Second, the ribonucleoprotein telomerase elongates shortened telomeres at chromosomal ends using a reverse transcriptase activity. Although the human telomerase holoenzyme is composed of multiple accessory subunits, catalysis is localized to the telomerase reverse transcriptase (TERT) subunit. We found that, in terms of global protein structure, minimal rearrangement is required to proceed through the catalytic cycle.

Throughout the TERT catalytic cycle, we observed that Y256 rests in the minor groove of the DNA and is in position to clash with the 2’-OH of an incoming rNTP. Therefore, we hypothesized this residue to be the steric gate in telomerase. Compared to WT TERT, the insertion of a matched rGTP by Y256A showed a 1,490-fold increase in kpol to 5.5 s−1 and a 12-fold decrease in Kd to 73 μM. Thus, the sugar selectivity of TERT dropped from 14,000-fold between rGTP and dGTP for WT TERT to less than 2-fold for the Y256A TERT variant. To test for structural rearrangements, we crystallized the pre-nucleotide binary state of TERT Y256A (state A6), and saw minimal structural differences compared to the WT protein. The position of the primer terminus was not changed, and catalytic residues D251, D343, and D344 were in position to catalyze the nucleotidyl transferase reaction. Upon closer examination of the active site pocket, the substitution of Y256 with alanine resulted in a more open nucleotide binding pocket. The distance from the C2 carbon of the dGpCpp to residue 256 shifted from 3.3 Å in WT TERT to 5.7 Å in TERT Y256A, showing that the TERT Y256A has much more room to accommodate the 2’-OH. Taken as a whole, these results indicate Y256 clashes with the 2’-OH of rNTPs to provide sugar discrimination and is the steric gate in telomerase.

> GMVHYYRLSLKSRQKAPKIVNSKYNSILNIALKNFRLCKKHKTKKPVQILALLQEIIPKSYFGTTTNLKRFYKVVEKILTQSSFECIHLSVLHKCYDYDAIPWLQNVEPNLRPKLLLKHNLFLLDNIVKPIIAFYYKPIKTLNGHEIKFIRKEEYISFESKVFHKLKKMKYLVEVQDEVKPRGVLNIIPKQDNFRAIVSIFPDSARKPFFKLLTSKIYKVLEEKYKTSGSLYTCWSEFTQKTQGQIYGIKVDIRDAAGNVKIPVLCKLIQSIPTHLLDSEKKNFIVDHISNQFVAFRRKIYKWNHGLLQGDPLSGCLCELYMAFMDRLYFSNLDKDAFIHRTVDDYFFCSPHPHKVYDFELLIKGVYQVNPTKTRTNLPTHRHPQDEIPYCGKIFNLTTRQVRTLYKLPPNYEIRHKFKLWNFNNQISDDNPARFLQKAMDFPFICNSFTKFEFNTVFNDQRTVFANFYDAMICVAYKFDAAMMALRTSFLVNDFGFIWLVLSSTVRAYASRAFKKIVTYKGGKYRKVTFQCLKSIAWRAFLAVLKRRTEIYKGLIDRIKSREKLTMKFHDGEVDASYFCKLPEKFRFVKINRKASI>GPMEEKALIGIEDFLKVDLRVAKVLSAERVEGSEKLLKLTLSLGDEERTVVAGIAKYYTPEELVGKKIVIVANLKPRKIFGIESQGMILAASDGENLSVIVPDRDVKEGAKLS[2x]

Across all domains of life, a widespread class of OB folds have specialized to recognize and manipulate tRNAs, perform key functions in tRNA trafficking and metabolism, and are designated as the tRNA binding domain (TRBD) superfamily (IPR002547; PF01588). In bacteria, Aquifex aeolicus Trbp111 (tRNA-binding protein, 111 amino acids) and Escherichia coli Trbp exemplify the free-standing, dimeric OB-fold proteins that bind diverse tRNA species. Trbp has been suggested to facilitate the folding of the tRNA structure by binding its characteristic elbow region formed by the intercalation of the D-loop into the T-loop and was observed to enhance aminoacylation by several aminoacyl-tRNA synthetases (aaRSs). Contrary to previous proposals, Trbp111 does not recognize the global tRNA structure nor its elbow or anticodon but solely binds its universal 3′ terminal single-stranded CA dinucleotide with a strong positional, structural, and sequence preference.

To confirm our in-solution finding that Trbp111 binds the tRNA 3′ end and to visualize the interface, we determined its co-crystal structure at 2.6 Å by engineering the tRNA ASL region which does not contribute to binding. We observed two tRNAs bound to a Trbp111 dimer in crystallo employing nearly identical interfaces, each burying ~ 484 Å2 of solvent-accessible surfaces. The structure reveals acute bending of the tRNA terminal dinucleotide (tC75-tA76) away from the tRNA body and its preceding single-stranded nucleotides (tA73, tC74). Comparing the two complexes in the asymmetric unit, the Trbp111-bound tC75-tA76 dinucleotide pivots relative to the tRNA body as a rigid body due to the flexible tA73-tC74 linker. Interestingly, tC75 and tA76 are independently recognized by two pre-formed sequence-selective binding pockets. The penultimate tC75 nucleobase forms a T-shaped π-π stacking interaction with F78 and is further anchored by hydrogen bonds from the backbone amide nitrogen atoms of E32 and K33. The immediately preceding tC74 is oriented away from the protein surface so as not to clash with F78. The terminal tA76 is captured by a predominantly hydrophobic pocket, with the nucleobase sandwiched by M85 on one side and the R75 methylene groups and I77 on the other. The tA76 nucleobase is further recognized by hydrogen bonds from S82 and the K73 carbonyl group. Single substitutions of evolutionarily conserved, interfacial Trbp111 residues impaired tRNA binding, with the largest defects from R75A nearly abolishing binding, followed by K33A, S82A, M85A, and F78A.> MSGSEEEKPIVIDLNKTIERDGRKVKLVRATITVDPETNTITIDIEYEGGPITKEDLLEAFK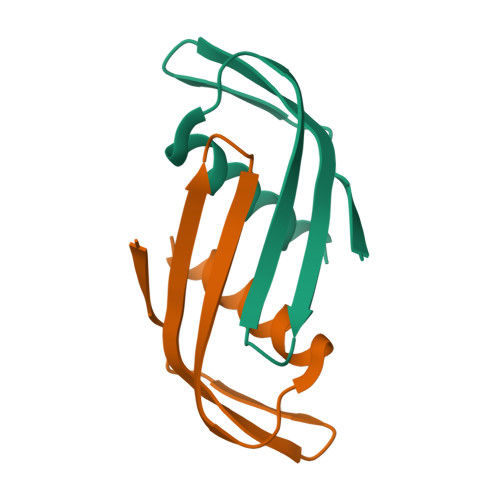LAASKLGS>[7x]MGHHHHHHHHHHSSGHIDDDD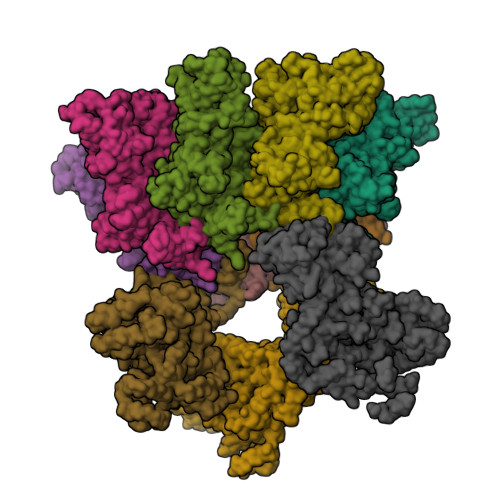KHMEVKQENRLLNESESSSQGLLGYYFSDLNFQAPMVVTSSTTGDLSIPSSELENIPSENQYFQSAIWSGFIKVKKSDEYTFATSADNHVTMWVDDQEVINKASNSNKIRLEKGRLYQIKIQYQRENPTEKGLDFKLYWTDSQNKKEVISSDNLQLPELKQKSSNSRKKRSTSAGPTVPDRDNDGIPDSLEVEGYTVDVKNKRTFLSPWISNIHEKKGLTKYKSSPEKWSTASDPYSDFEKVTGRIDKNVSPEARHPLVAAYPIVHVDMENIILSKNEDQSTQNTDSQTRTISKNTSTSRTHTSEVHGNAEVHASFFDIGGSVSAGFSNSNSSTVAIDHSLSLAGERTWAETMGLNTADTARLNANIRYVNTGTAPIYNVLPTTSLVLGKNQTLATIKAKENQLSQILAPNNYYPSKNLAPIALNAQDDFSSTPITMNYNQFLELEKTKQLRLDTDQVYGNIATYNFENGRVRVDTGSNWSEVLPQIQETTARIIFNGKDLNLVERRIAAVNPSDPLETTKPDMTLKEALKIAFGFNEPNGNLQYQGKDITEFDFNFDQQTSQNIKNQLAELNATNIYTVLDKIKLNAKMNILIRDKRFHYDRNNIAVGADESVVKEAHREVINSSTEGLLLNIDKDIRKILSGYIVEIEDTEGLKEVINDRYDMLNISSLRQDGKTFIDFKKYNDKLPLYISNPNYKVNVYAVTKENTIINPSENGDTSTNGIKKILIFSKKGYEIG;>[3x]MNIKKEFIKVISMSCLVTAITLSGPVFIPLVQGAGGHGDVGMHVKEKEKNKDENKRKDEERNKTQEEHLKEIMKHIVKIEVKGEEAVKKEAAEKLLEKVPSDVLEMYKAIGGKIYIVDGDITKHISLEALSEDKKKIKDIYGKDALLHEHYVYAKEGYEPVLVIQSSEDYVENTEKALNVYYEIGKILSRDILSKINQPYQKFLDVLNTIKNASDSDGQDLLFTNQLKEHPTDFSVEFLEQNSNEVQEVFAKAFAYYIEPQHRDVLQLYAPEAFNYMDKFNEQEINLSLEELKDQRMLARYEKWEKIKQHYQHWSDSLSEEGRGLLKKLQIPIEPKKDDIIHSLSQEEKELLKRIQIDSSDFLSTEEKEFLKKLQIDIRDSLSEEEKELLNRIQVDSSNPLSEKEKEFLKKLKLDIQPYDINQRLQDTGGLIDSPSINLDVRKQYKRDIQNIDALLHQSIGSTLYNKIYLYENMNINNLTATLGADLVDSTDNTKINRGIFNEFKKNFKYSISSNYMIVDINERPALDNERLKWRIQLSPDTRAGYLENGKLILQRNIGLEIKDVQIIKQSEKEYIRIDAKVVPKSKIDTKIQEAQLNINQEWNKALGLPKYTKLITFNVHNRYASNIVESAYLILNEWKNNIQSDLIKKVTNYLVDGNGRFVFTDITLPNIAEQYTHQDEIYEQVHSKGLYVPESRSILLHGPSKGVELRNDSEGFIHEFGHAVDDYAGYLLDKNQSDLVTNSKKFIDIFKEEGSNLTSYGRTNEAEFFAEAFRLMHSTDHAERLKVQKNAPKTFQFINDQIKFIINS>GPLGRGREEKAPEEPQPVKMPENNSVVEATWNDVQLEDSLGMEVGYRLIPMVDFQQDGELLGRIRSIRKKFAQDMGFLPPVVHIRDNMDLQPARYRILMKGVEIGSGDAYPGRWLAINPGTAAGTLPGEKTVDPAAGLDAIWIESALKEQAQIQGFTVVEASTVVATHLNHLIGQFSAELFGRQEAQQLLDRVSQEMPKLTEDLVPGVVTLTTLHKVLQNLLAEKVPIRDMRTILETLAEHAPLQSDPHELTAVVRVALGRAITQQWFPG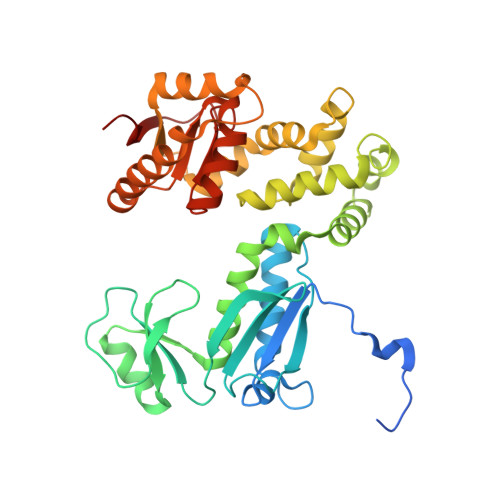NEEVQVIGLDTALERLLLQALQGGGGLEPGLADRLLAQTQEALSRQEMLGAPPVLLVNHALRPLLSRFLRRSLPQLVVLSNLELSDNRHIRMTATIGGK[2x]> MKHHHHHHHGAAGTSLY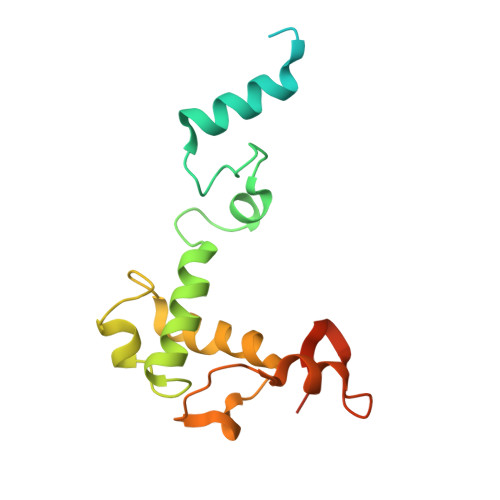KKAGENLYFQGSMKKNGKSQNQPLDFTQYAKNMRKDLSNQDICLEDGALNHSYFLTKKGQYWTPLNQKALQRGIELFGVGNWKEINYDEFSGKANIVELELRTCMILGINDITEYYGKKISEEEQEEIKKSNIAKGKKENKLKDNIYQKLQQMQ> GSMASAPLRVYVQCNPLLDVSAHVSDEFLVKYGLERGTAILLSERQKGIFDDIEKMPNVRYVPGGSGLNVARVAQWMQQAYKGKFVTYVGCIADDRYGKVLKEAAEHEGIVMAVEHTTKAGSGACAVCITGKERTLVADLGAANHLSSEHMRSPAVVRAMDESRIFYFSGFTLTVDVNHVLQACRKAREVDGLFMINLSAPFIMQFFSAQLGEVLPYTDIIVANRHEAKEFANMMKWDTDCVEEIARRAVSEVPYTGTKGRVVVFTRDIESTVLATKDGVETVPVPQLDQDKVIDMNGAGDAFMGGFLSAYAVGKDLRRCCETGHYTAQEVIQRDGCSFPEKPSFSP

Adenosine kinase (EC 2.7.1.20, ATP:adenosine 5′-phosphotransferase) catalyzes the phosphorylation of adenosine to adenosine monophosphate (AMP) in presence of Mg2+ and utilizing ATP as the preferred phosphoryl donor. Recently T. brucei adenosine kinase (TbAK) was identified as a key enzyme mediating high affinity adenosine salvage in the purine salvage pathway. The overall structures of both TbrAK in complex with AP5A and compound 1 contain a mixed fold and consist of 12 α-helices and 14 β-strands that form two distinct domains. A common property of adenosine kinases from various organisms is their control via substrate-inhibition to prevent non-physiologically high intracellular purine nucleotide levels, and recently it has been shown that TbrAK activity is strongly inhibited by its substrate adenosine.

However, the diffraction from one of the apo crystals that had been soaked with compound 1, while still exhibiting several overlapping lattices indicative of non-merohedral twinning, was of sufficient quality to allow indexing of a single lattice, yielding data of sufficient quality for model refinement to at resolution of 2.8 Å. The crystal system was found to be tetragonal with space group P41212 with one molecule in the asymmetric unit and without any contacts other than typical crystal contacts with neighboring molecules in the crystal lattice. TbrAK in complex with compound 1 adopts an open conformation, and the location of compound 1 was unambiguously identified by its well-defined electron density localized in part in the adenosine binding site in the adenine moiety binding area, but pointing away from the ribose binding region towards the solvent. Moreover, only this orientation satisfies a number of hydrogen bonds to the protein, supporting the conclusion that compound 1 binds to TbrAK with the phenoxyphenyl moiety pointing towards the outside and the morpholine being buried in the active site. Compound 1 forms three hydrogen bonds with the protein, namely with the side chain NH2 groups of N13 and N142 (water-mediated) and the main chain nitrogen of S64. The phenoxy moiety of compound 1 interacts mainly via hydrophobic contacts formed by F169, F200, F204 and F205. Thus compound 1 is able to induce the formation of the anion hole also in absence of ATP, which could favor ATP rather than adenosine binding in the ATP binding pocket due to favorable interactions with the β and γ phosphate groups. As a result, the intrinsic substrate inhibition would be abolished, which corresponds exactly to the recent observation of abolishment of substrate inhibition conferred by compound 1 towards TbrAK. As compound 1 is not strongly interacting with the lid domain, it is most probably not able to interfere with the hinge bending motion to close the lid domain.> MKKVGNHNSISRKLLLSLSLTLIFSLTSFAQDPAAAPAATEAAAPAAASGGDPVKGKELFNANCAACHKLDAKSTGPALRGVASKHDMAWIYKWVHNSSDMIKSGDPVAVKLFEENNKAVMTSFPQLSTGDIDNIIAYTSEVKAEPAAAAGGAATPPGTNVEGGGISNNIILGALALVMAILVVMLFMVNKVLTKVASNNGIEVAPKEGRTPIWKAFAKNQFLVLVTSIFLLLASGYFVYGYLMQVGVDQNYEPIQPIHYSHKIHAGDNEINCKYCHSAARVSKTAGIPSLNVCMNCHKNISEVAETTATAEYSKAFYDAQIQKLYDAVGWDKTKQAYTGKTQPVKWVRIHNLPDFVYFNHSQHVSVAGVECQTCHGPVQEFEIMKQYSKLTMGWCVDCHRKTDVKMEGNAYYEKIHAE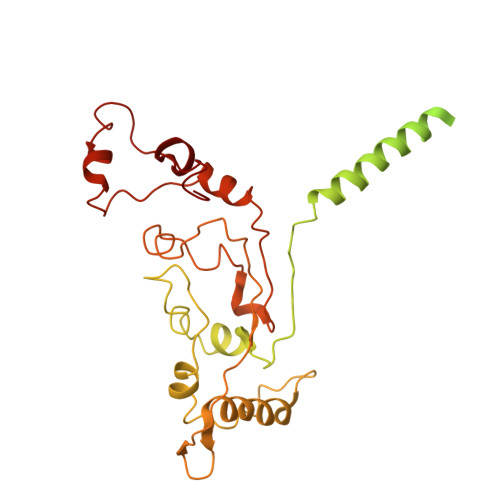LSKKYGVEKLTAAQMGGLECGKCHY>SLGLLKAFNNFPITNKIQCNGLFTPSNIETLLGGTEIGKFTVTPKSSGSMFLVSADIIASRMEGGVVLALVREGDSKPCAISYGY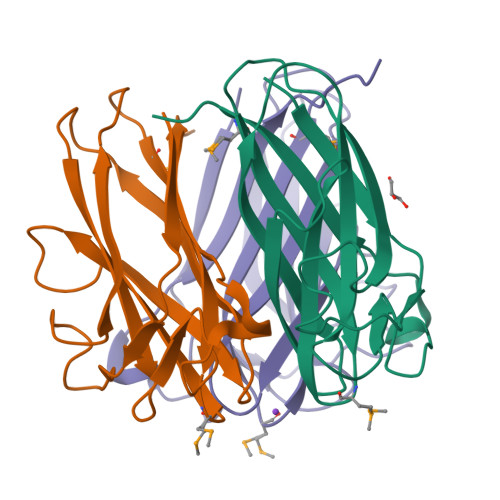SSGVPNLCSLRTSITNTGLTPTTYSLRVGGLESGVVWVNALSNGNDILGITNTSNVSFLEVIPQTNA[3x]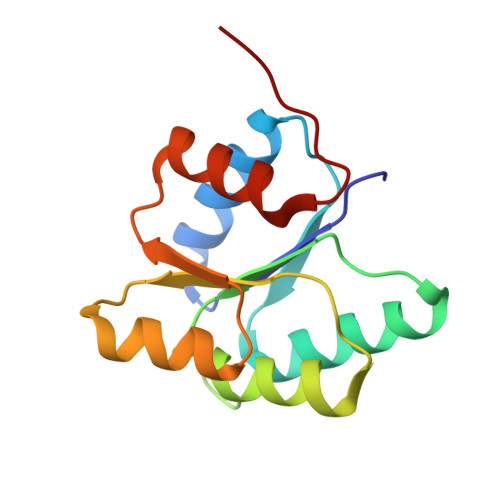> TSVKILVVEDNHVNQEVIKRMLNLEGIENIELACDGQEAFDKVKELTSKGENYNMIFMDVQMPKVDGLLSTKMIRRDLGYTSPIVALTAFADDSNIKECLESGMNGFLSKPIKRPKLKTILTEFCAAYQGKKN9-(N,N-DIMETHYLGLYCYLAMIDO)-6-DEOXY-6-DEMETHYL-TETRACYCLINE 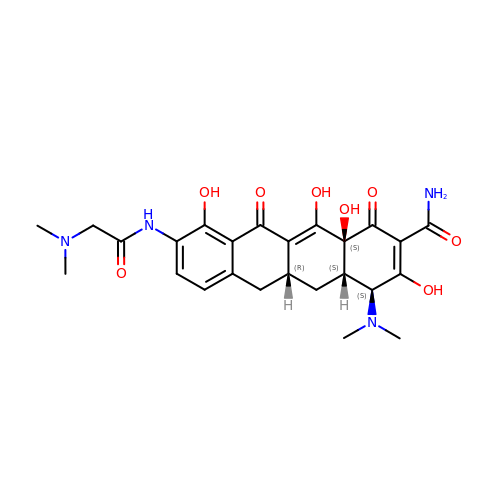| C25 H30 N4 O8 | OAZYAPOSQALFER-CLPWGHEBSA-N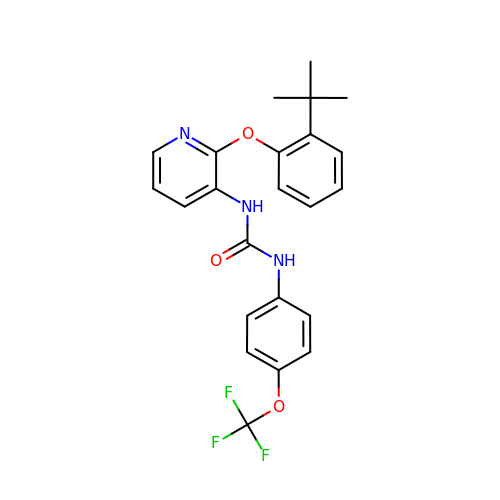1-[2-(2-tert-butylphenoxy)pyridin-3-yl]-3-[4-(trifluoromethoxy)phenyl]urea | C23 H22 F3 N3 O3 | AHFLGPTXSIRAQK-UHFFFAOYSA-N>[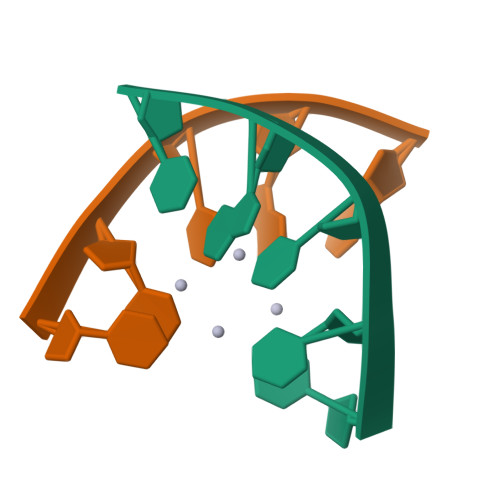24x]TTTGC>[2x]NSMIDKFCDWFEGEFDNWTQAASNPTKWAHIIVKHEKISEYKYHTSSRYSYMDKPYREQTVDIEYVCPELIIVHNPACDIIFKWTGIYFEGESEPDC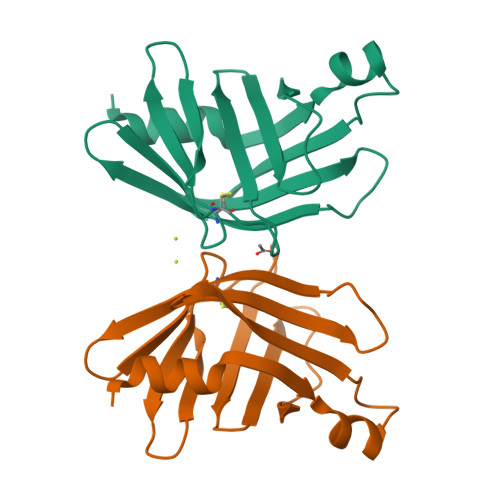QWNGQPLDSKARLYADEYHTWDVGYWEGSEGFFHFKKNV>SGGGLPSTVIAISYFEGFVKLAAEWIVTEMPTTEIDGKTYTSGKLYIKMPETLDTDIKKSAMLFYKKQGLNETQMSTNHRNYPIHIVSKEEGDTLEVYDMPTILSGIDKAIDMYFRVGHIGKTTEQQLAEDNEMNNFKRVLQLLINEDSFCRECVEILRQA[2x]

During phage infection, bacterial STING sense c-di-GMP generated by the CD-NTase (cGAS/DncV-like nucleotidyltransferase) encoded in the same operon and signal suicide commitment as a defense strategy that restricts phage propagation. The structure of MySTING was then solved by MR using the refined model of PcSTING. Both PcSTING and MySTING crystals contained two nearly identical protomers with root-mean-square deviations (RMSDs) of 0.29 Å and 0.64 Å for 158 and 160 matched Cα pairs in the asymmetric unit, forming canonical V-shaped dimers of STING domain. Here, our structures demonstrate that the symmetric recognition of single c-di-GMP by dimeric bacterial STING proteins is dictated by the guanidinium group of arginine residue (R233/R230 in PcSTING/MySTING) that recognizes the O6 and N7 atoms of guanine base, the backbone oxygen and amide group (H238/H235 in PcSTING/MySTING) that form three hydrogen bonds to the Watson-Crick edge of guanine base and the aspartate residue (D252/D251 in PcSTING/MySTING) that binds to the N2 atom of guanine base.

We turned to prepare SeMet-labeled PcSTING and solved the structure at 2.25-Å resolution. Although no nucleotide was included in the crystallization solution, the strong electron-density unambiguously identified the bound CDN as c-di-GMP. In addition to the specific H-bonding interaction, each guanine base of c-di-GMP is sandwiched by extensive π–π stacking interaction formed by F171 of one PcSTING protomer and Y235 of the other protomer. The planar guanidinium group of R233 also stacks with the aromatic ring of Y235, forming a unique Phe/Guanine/Tyr/Arg four-layer stack buttressed by the four H-bond interactions between R233 and c-di-GMP. By contrast, in PcSTING/MySTING the stacking interaction of R233/R230 and Y235/Y232 locks the conformation of the guanidinium group of R233/R230 into specific hydrogen bonds with the O6 and N7 atoms of c-di-GMP. Moreover, mutating the specificity-determining residue D252 or R233 in PcTIR-STING relieved the growth inhibition, validating the importance of these two residues in recognition of c-di-GMP. Each V-shaped dimer of PcSTING associates with its neighbors on both sides, which are symmetry-related by unit-cell translation along the c axis. The small helix α5 interacts with helix α2 of the other dimer by both hydrophobic and ionic interactions including two salt-bridges (K212–D301, K220–E306), one hydrogen bond (S213–S302), and the close side-chain packing of F303, K212, M215, and L216. The loop connecting helix α3 and α4 (denoted 3–4 loop, residues 267–276) in PcSTING intercalated into a groove formed by helix α1 and α4 of protomer A’ and the 3–4 loop of protomer B’ of the other dimer. The interactions are mediated mainly by the protein backbone with additional side-chain contacts of I273 and M266.> QTAR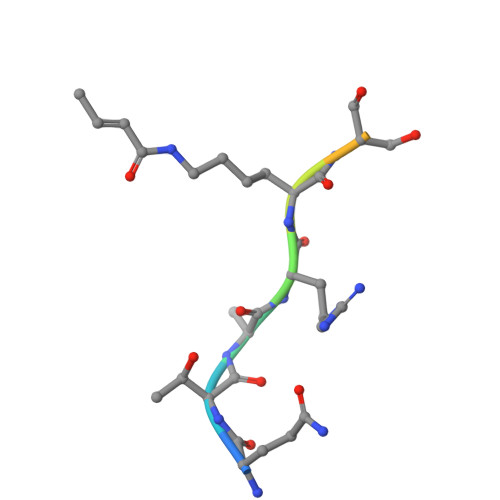XSSTGG3-[cis-3-(4-methylpiperazin-1-yl)cyclobutyl]-1-(2-phenylquinolin-7-yl)imidazo[1,5-a]pyrazin-8-amine | C30 H31 N7 | 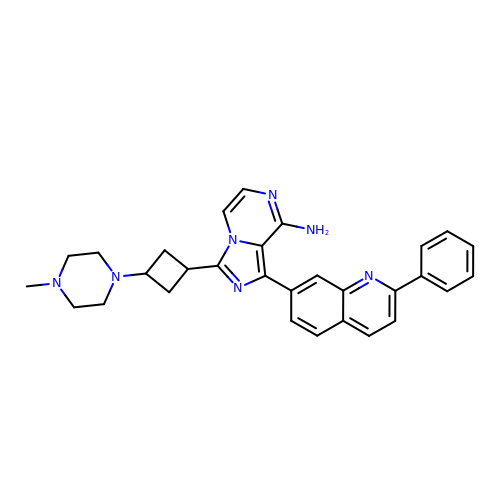PDJARQSWGDDFHH-PSWAGMNNSA-N N-[2-(1,3-BENZODIOXOL-5-YL)ETHYL]-1-[2-(1H-IMIDAZOL-1-YL)-6-METHYLPYRIMIDIN-4-YL]-D-PROLINAMIDE | C22 H24 N6 O3 | 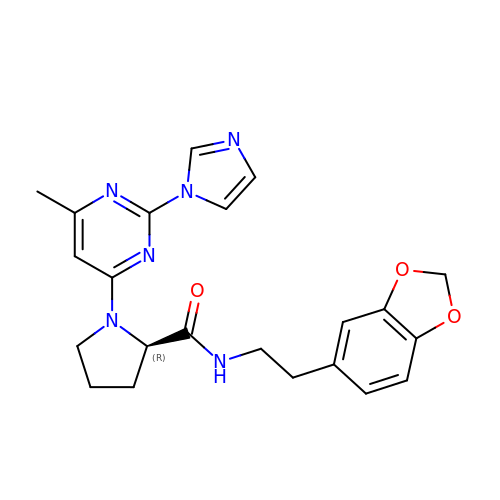LBCGUKCXRVUULK-QGZVFWFLSA-N>SNAMNSQLTLRALERG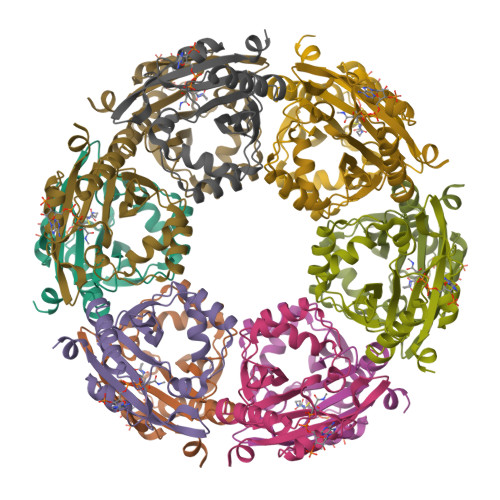DLRFIHNLNNNRNIMSYWFEEPYESFDELEELYNKHIHDNAERRFVVEDAQKNLIGLVELIEINYIHRSAEFQIIIAPEHQGKGFARTLINRALDYSFTILNLHKIYLHVAVENPKAVHLYEECGFVEEGHLVEEFFINGRYQDVKRMYILQSKYLNRSE[12x]> MIIYGVYIVSKSGGLIFNLDNNVPRIEHEKTFTYPLDLVLDYDSKKVSVSFNRKDGINVGHVLVAVNGMPVNGVTLDDGRDVRTTLDAPENYPINLKFSRPKMTTNEKIFLASMFYPLFAIASQLSPEPKSSGIEILEADTFTLHCF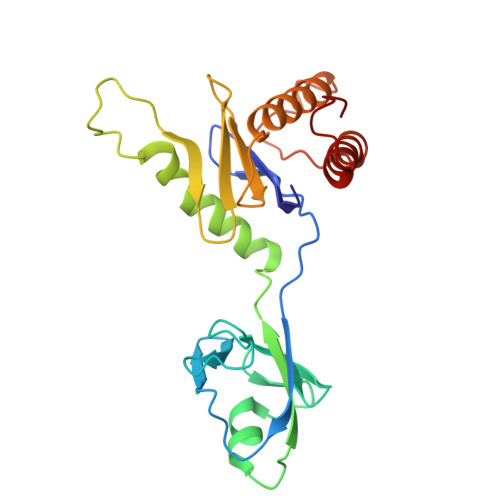QTLTGIKFIIISETGLNGIDLLLRKVYELYSDYVLKNPFYSLEMPIRCELFDNKLQELLAQVEKTGISNIDK>[2x]MRSRRVDVMDVMNRLILAMDLMNRDDALRVTGEVREYIDTVKIGYPLVLSEGMDIIAE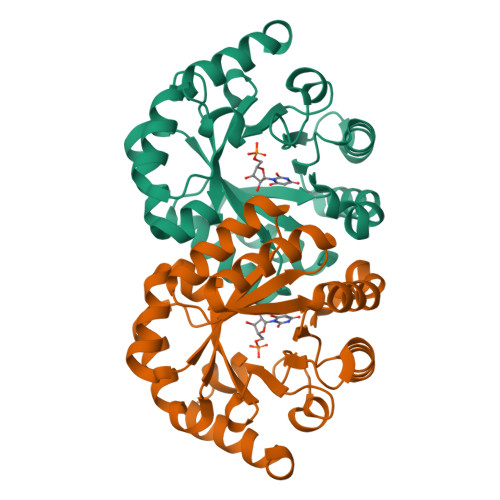FRKRFGCRIIADFKVADIPETNEKICRATFKAGADAIIVHGAPGADSVRACLNVAEEMGREVFLLTEMSHPGAEMFIQGAADEIARMGVDLGVKNYVGPSTRPERLSRLREIIGQDSFLISPGVGAQGGDPGETLRFADAIIVGRSIYLADNPAAAAAGIIESIKDLLNP>MNPAAEAEFNILLATDSYKVTHYKQYPPNTSKVYSYFECREKKTENSKLRKVKYEETVFYGLQYILNKYLKGKVVTKEKIQEAKDVYKEHFQDDVFNEKGWNYILEKYDGHLPIEIKAVPEGFVIPRGNVLFTVENTDPECYWLTNWIETILVQSWYPITVATNSREQKKILAKYLLETSGNLDGLEYKLHDFGYRGVSSQETAGIGASAHLVNFKGTDTVAGLALIKKYYGTKDPVPGYSVPAAEHSTITAWGKDHEKDAFEHIVTQFSSVPVSVVSDSYDIYNACEKIWGEDLRHLIVSRSTQAPLIIRPDSGNPLDTVLKVLEILGKKFPVTENSKGYKLLPPYLRVIQGDGVDINTLQEIVEGMKQKMWSIENIAFGSGGGLLQKLTRDLLNCSFKCSYVVTNGLGINVFKDPVADPN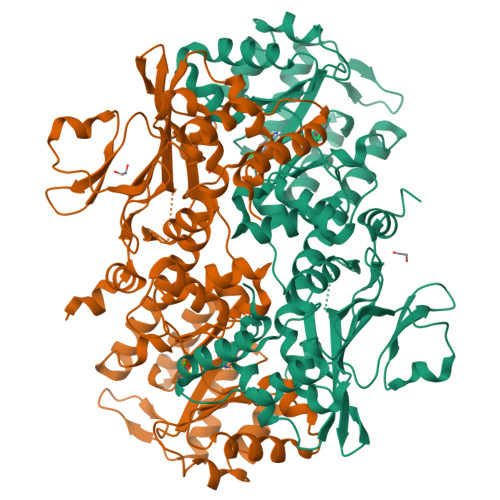KRSKKGRLSLHRTPAGNFVTLEEGKGDLEEYGQDLLHTVFKNGKVTKSYSFDEIRKNAQLNIELEAAHHLEHHHHHHHH[2x]> GSHMESGYAQNGDLEDAELDDYSFSCYSQLEVNGSQHSLTCAFEDPDVNTTNLEFEICGALVEVKCLNFRKLQEIYFIETKKFLLIGKSNICVKVGEKSLTCKKIDLTTIVKPEAPFDLSVVYREGANDFVVTFNTSHLQKKYVKVLMHDVAYRQEKDENKWTHVNLSSTKLTLLQRKLQPAAMYEIKVRSIPDHYFKGFWSEWSPS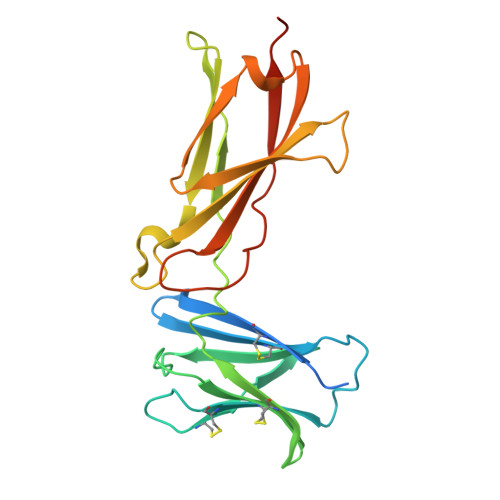YYFRTPEINNSSGEMD> VDCSEYPKPAC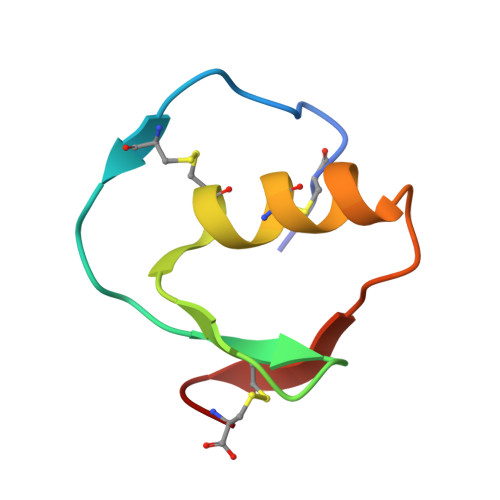TREYRPLCGSDNKTYGNKCNFCNAVVESNGTLTLSHFGKC>[2x]MTDNKRPQLKDKEPAAKPARTRKPKNETVALVVEATTEAEAKKSLREGGLVPAAHEIMIPVGNMILA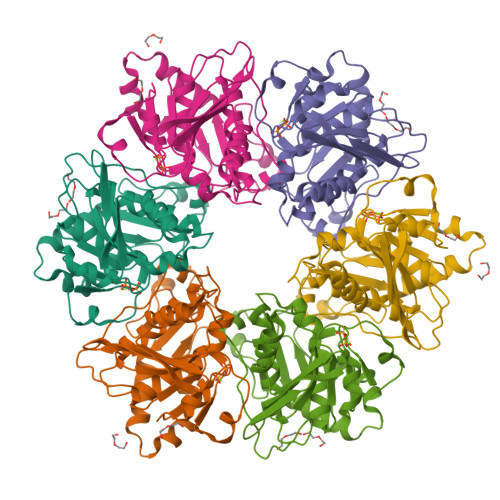VDTQVLDKCALALAASDDPGRWFAENESLIHSTVFAPVAKGLHRVYPLLSVRPEVPAGYEASWPTQDHMPGLHLVVGGTGAGKSSYLASQDLTLVIRWGEPAERFDVEGATHAVSDLNEALAVAFVMARAGYRPAIDSFRNLVFGIESAAGEGGISTALYSAMTAINNVCSRLGIVVMVVVNPMATEAKAELVYNNMAASVAGMTVLMDGAVSKQTVRTLSGRTWGVGKQPKAAVTEEVIPRATVVPQPSAVVRNTRLESQTIDVSDDDLNNEPGRQGSRKHI> MNPNQKIITIGSVCMTIGMANLILQIGNIISIWISHSIQLGNQNQIETCNQSVITYENNTWVNQTYVNISNTNFAAGQSVVSVKLAGNSSLCPVSGWAIYSKDNSIRIGSKGDVFVIREPFISCSPLECRTFFLTQGALLNDKHSNGTIKDRSPYRTLMSCPIGEVPSPYNSRFESVAWSASACHDGINWLTIGISGPDNGAVAVLKYNGIITDTIKSWRNNRLRTQESECACVNGSCFTVMTDGPSDGQASYKIFRIEKGKIVKSVEMNAPNYHYEECSCYPDSSEITCVCRDNWHGSNRPWVSFNQNLEYQIGYICSGIFGDNPRPNDKTGSCG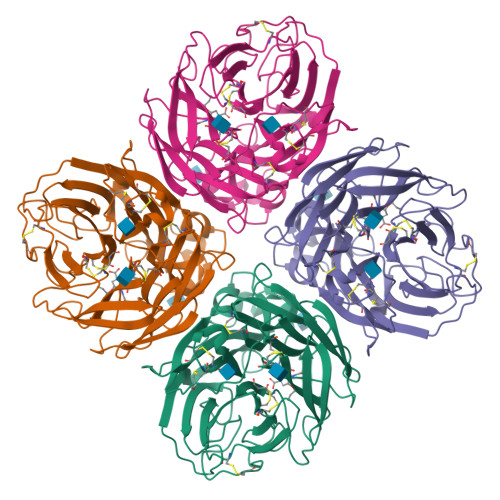PVSSNGANGVKGFSFKYGNGVWIGRTKSISSRNGFEMIWDPNGWTGTDNDFSIKQDIVGINEWSGYSGSFVQHPELTGLDCIRPCFWVELIRGRPKENTIWTSGSSISFCGVNSDTVGWSWPDGAELPFTIDK>[2x]GFARLKRSLLKTKENLGSGFISLFRGKKIDDDLFEELEEQLLIADVGVETTRKIITNLTEGASRKQLRDAEALYGLLKEEMGEILAKVDEPLNVEGKAPFVILMVGVNGVGKTTTIGKLARQFEQQGKSVMLAAGDTFRAAAVEQLQVWGQRNNIPVIAQHTGADSASVIFDAIQAAKARNIDVLIADTAGRLQNKSHLMEELKKIVRVMKKLDVEAPHEVMLTIDASTGQNAVSQAKLFHEAVGLTGITLTKLDGTAKGGVIFSVADQFGIPIRYIGVGERIEDLRPFKADDFIEALFARED

The signal recognition particle (SRP) is an efficient protein sorting system that directs the translocation of newly synthesized proteins from translating ribosomes to the endoplasmic reticulum (ER) or plasma membrane. Similarly, the eukaryotic SRP receptor (SR) consists of two proteins, SRα and the membrane-inserted SRβ, while in bacteria, a single protein, FtsY, is responsible for membrane association and interaction with the translocon. In FtsY, the NG domain (comprising of the N-terminal and GTP binding domains) is involved in binding a GTP molecule and forming a heterodimer with the NG domain of Ffh. The N domain of FtsYNG consists of a four-helix bundle (αN1−N4), while the G domain adopts a classical Ras GTPase fold in which five conserved motifs (G1−G5) are arranged around the nucleotide-binding site.

Apo FtsYNG crystals diffracted to 1.45Å with two copies of the protein in the asymmetrical unit. The structures show the N domain of one monomer packing against the G domain of the other copy in the asymmetric unit. Also an unique αβαβ domain to the SRP GTPase family named Insertion Box Domain (IBD) is present in the G domains and is involved in 4.5S RNA recognition and interaction with Ffh as previously reported. The apo structure was then used as a search model for all subsequent FtsYNG:fragment structures (herein referred to as holo structures) using molecular replacement.> GCGGCA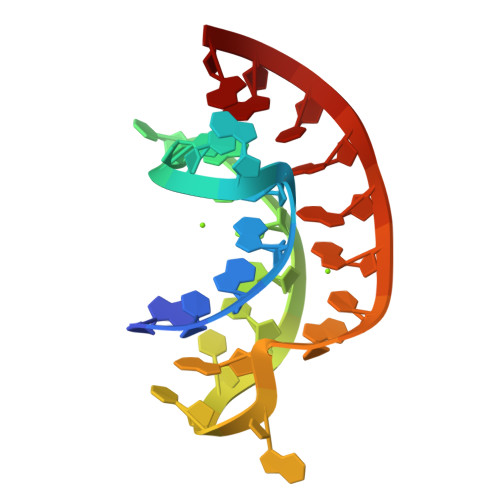CCGUCCGCUCAAACAAACGG> SEELEKALSKLSEREAMVLKLRKGLIDGREHTLEEVGAYFGVTRERIRQIENKA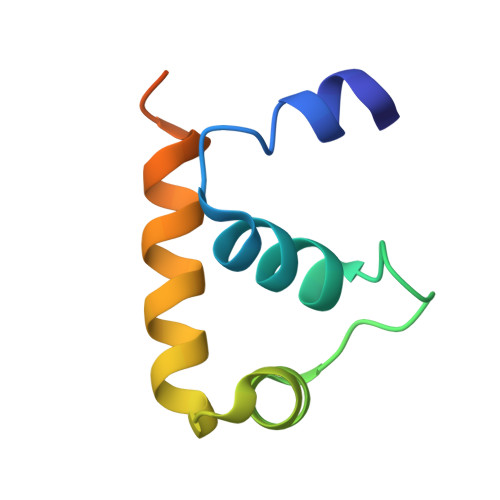LRKLKYHESRTRKLRDFLE>SNAAKDVKFGADARALMLQGVDLLADAVAVTMGPKGRTVIIEQSWGSPKVTKDGVTVAKSIDLKDKYKNIGAKLIQDVANNTNEEAGDGTTTATVLARSIAKEGFEKISKGANPVEIRRGVMLAVDAVIAELKKQSKPVTTPEEIAQVATISANGDKEIGNIISDAMKKVGRKGVITVKDGKTLNDELEIIEGMKFDRGYISPYFINTSKGQKCEFQDAYVLLSEKKISSIQSIVPALEIANAHRKPLVIIAEDVDGEALSTLVLNRLKVGLQVVA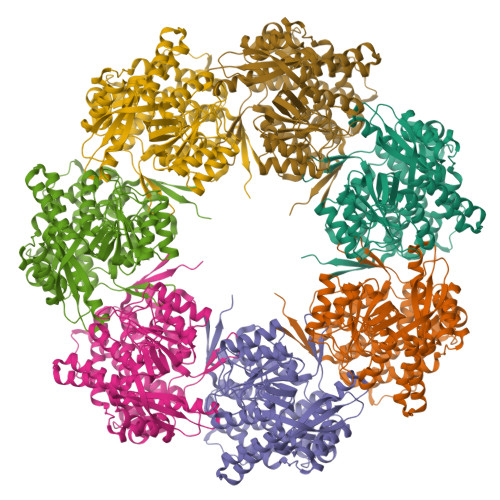VKAPGFGDNRKNQLKDMAIATGGAVFGEEGLTLNLEDVQPHDLGKVGEVIVTKDDAMLLKGKGDKAQIEKRIQEIIEQLDVTTSEYEKEKLNERLAKLSDGVAVLKVGGTSDVEVNEKKDRVTDALNATRAAVEEGIVLGGGCALLRCIPALDSLTPANEDQKIGIEIIKRTLKIPAMTIAKNAGVEGSLIVEKIMQSSSEVGYDAMAGDFVNMVEKGIIDPTKVVRTALLDAAGVASLLTTAEVVVTEIPKEEKDPGMGAMGGMGGGMGGGMF[7x]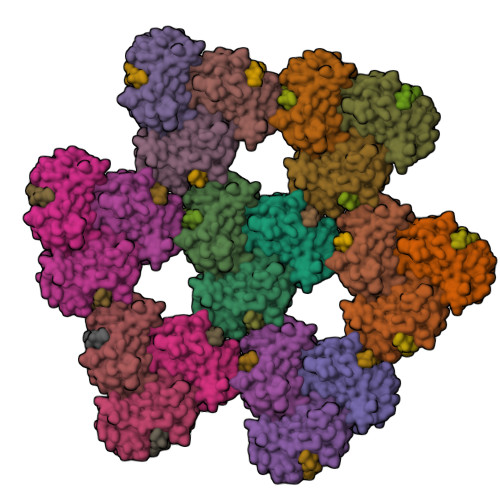>MSNSLEKKVSLLQNESVEKNKSIQSLHNQICSFEIEIERQKEMLRNNESKILHLQRVIDSQAEKLKELDKEIRPFRQNWEEADSMKSSVESLQNRVTELESVDKSAGQVARNTGLLESQLSRHDQMLSVHDIRLADMDLRFQVLETASYNGVLIWKIRDYKRRKQEAVMGKTLSLYSQPFYTGYFGYKMCARVYLNGDGMGKGTHLSLFFVIMRGEYDALLPWPFKQKVTLMLMDQGSSRRHLGDAFKPDPNSSSFKKPTGEMNIASGCPVFVAQTVLENGTYIKDDTIFIKVIVDTSDLPDPGGSLVPR[21x];>[21x]MRRGPRSLRGRDAPAPTPCVPAECFDLLVRHCVACGLLRTPRPKPAGASSPAPRTALQPQESVGAGAGEAALPLPGLLFGAPALLGLALVLALVLVGLVSWRRRQRRLRGASSAEAPDGDKDAPEPLDKVIILSPGISDATAPAWPPPGEDPGTTPPGHSVPVPATELGSTELVTTKTAGPEQQSNSLEVLFQ>[2x]MTMDEQQSQAVAPVYVGGFLARYDQSPDEAELLLPRDVVEHWLHAQGQGQPSLSVALPLNINHDDTAVVG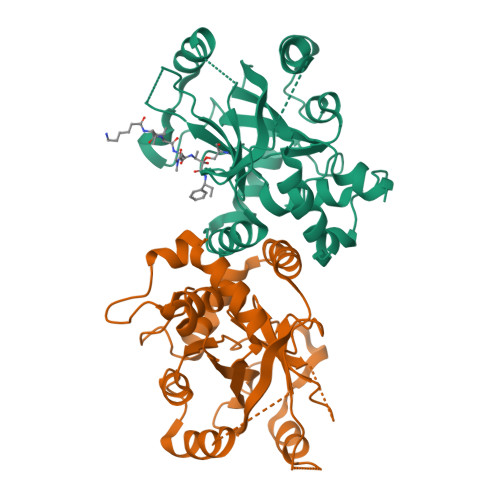HVAAMQSVRDGLFCLGCVTSPRFLEIVRRASEKSELVSRGPVSPLQPDKVVEFLSGSYAGLSLSSRRCDDVEQATSLSGSETTPFKHVALCSVGRRRGTLAVYGRDPEWVTQRFPDLTAADRDGLRAQWQRCGSTAVDASGDPFRSDSYGLLGNSVDALYIRERLPKLRYDKQLVGVTERESYVKA3-{8-[(3,4-dimethoxyphenyl)amino]imidazo[1,2-a]pyrazin-6-yl}benzamide 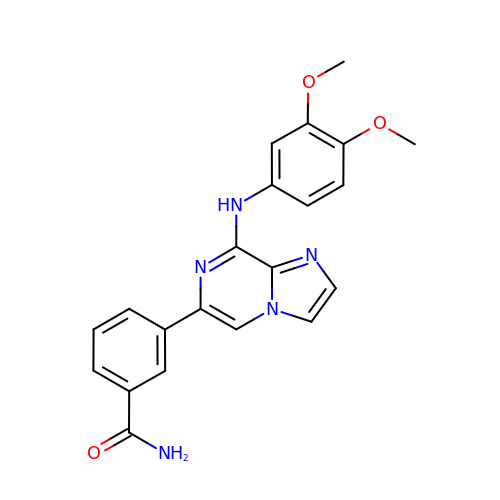| C21 H19 N5 O3 | QJHCMTUHZIJSPR-UHFFFAOYSA-N>[4x]GGGGGPGELGKPVRLPKEMSDEMKKAVDDGWTKNAFNQYVSDLISVHRTLPDPRDAWCKDEARYLTNL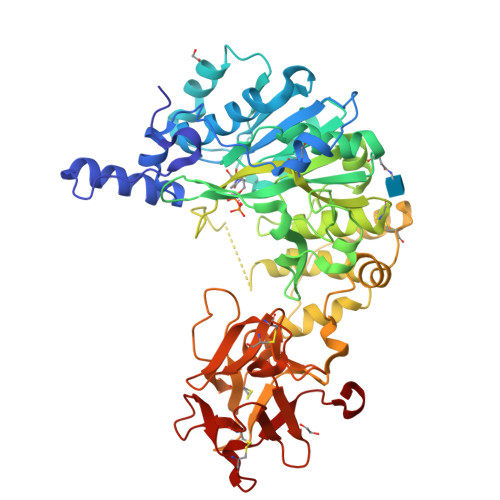PKTDVIICFHNEAWTVLLRTVHSVLDRSPEHLIGKIILVDDYSDMPHLKRQLEDYFAAYPKVQIIRGQKREGLIRARILGANHAKSPVLTYLDSHCECTEGWLEPLLDRIARNSTTVVCPVIDVISDETLEYHYRDSGGVNVGGFDWNLQFSWHPVPERERKRHNSTAEPVYSPTMAGGLFSIDREFFDRLGTYDSGFDIWGGENLELSFKTWMCGGTLEIVPCSHVGHIFRKRSPYKWRSGVNVLKKNSVRLAEVWMDEYSQYYYHRIGNDKGDWGDVSDRRKLRNDLKCKSFKWYLDNIYPELFIPGDSVAHGEIRNLGYGGRTCLDAPAGKKHQKKAVGTYPCHRQGGNQYWMLSKAGEIRRDDSCLDYAGKDVTLFGCHGGKGNQFWTYRENTKQLHHGTSGKCLAISESKDKLLMEECSASLSRQQWTLENYDSSKL>[2x]MRGSHHHHHHGSASFLKKTMPFKTTIEGTVNGHYFKCTGK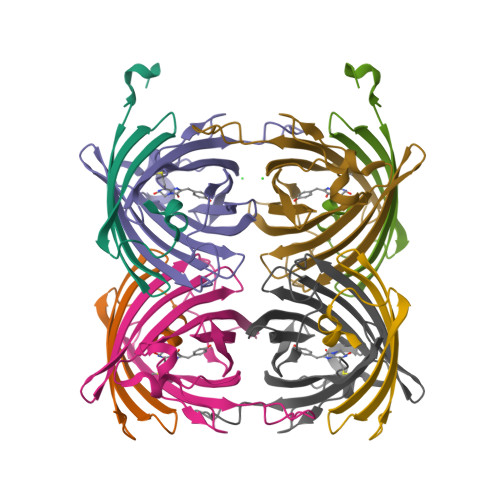GEGNPFEGTQEMKIEVIEGGPLPFAFHILSTSC;>MYGSKTFIKYVSGIPDYFKQSFPEGFTWERTTTYEDGGFLTAHQDTSLDGDCLVYKVKILGNNFPADGPVMQNKAGRWEPSTEIVYEVDGVLRGQSLMALKCPGGRHLTCHLHTTYRSKKPASALKMPGFHFEDHRIEIMEEVEKGKCYKQYEAAVGRYCDAAPSKLGHN[2x]>PGIHMQIGWRREGIKYRRNELFLDVLESVNLLMSPQGQVLSAHVSGRVVMKSYLSGMPECKFGMNDKIVIEKQGKGTADETSKSGKQSIAIDDCTFHQCVRLSKFDSERSISFIPPDGEFELMRYRTTKDIILPFRVIPLVREVGRTKLEVKVVIKSNFKPSLLAQKIEVRIPTPLNTSGVQVICMKGKAKYKASENAIVWKIKRMAGMKESQISAEIELLPTNDKKKWARPPISMNFEVPFAPSGLKVRYLKVFEPKLNYSDHDV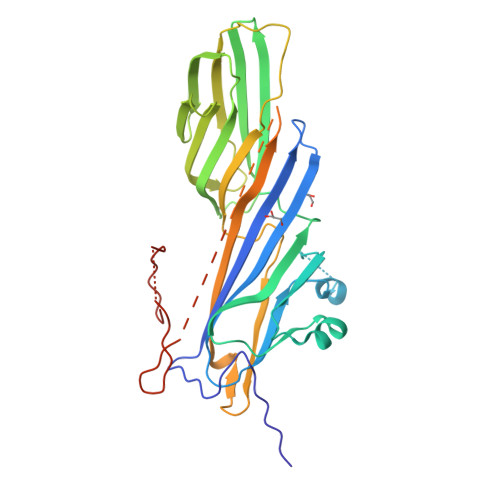IKWVRYIGRSGIYETRCGASGSAGSAGPSGAGSAGSAGPSAGSAGSAGSGSAGSAPGPDVDEEGYSIKPETNQNDTKENHFYSSSDSDSEDEE[2x]> MSKVFIATANAGKAHDADIFSVSACNSFTVSCSGDGYLKVWDNKLLDNENPKDKSYSHFVHKSGLHHVDVLQAIERDAFELCLVATTSFSGDLLFYRITREDETKKVIFEKLDLLDSDMKKHSFWAL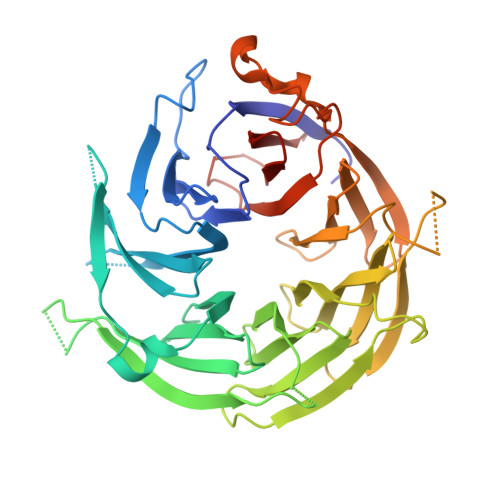KWGASNDRLLSHRLVATDVKGTTYIWKFHPFADESNSLTLNWSPTLELQGTVESPMTPSQFATSVDISERGLIATGFNNGTVQISELSTLRPLYNFESQHSMINNSNSIRSVKFSPQGSLLAIAHDSNSFGCITLYETEFGERIGSLSVPTHSSQASLGEFAHSSWVMSLSFNDSGETLCSAGWDGKLRFWDVKTKERITTLNMHCDDIEIEEDILAVDEHGDSLAEPGVFDVKFLKKGWRSGMGADLNESLCCVCLDRSIRWFREAGGK> MSVPSLEYQKQYIYSMQKSQCSIQNQSINIIADEQQAPQESYLSRKCQRHLFETKCVQLELGLNGDYSLSNNSLFIQNNNTVFDNLQQNTESNIKQTNRSNKERYETQIFEQHPIIKNPKNDQVSSIMNEQEQKKFINTDENVQQTAQVSKNSKQSFKNGIQQVQTLSIDKSQASIREQKKISDCNLDKQFIKGDSRLDESSKIPSKCCGWIPEDIIFENNIHQLNKKVTLVAKNNFSDSKIQNHKEKKYQQNFQKAAEIVNRLLNTSMNRIMRVRQHVRNFIMLLKLRYLNRKIDDLTDRDYASINDLSNFYKSHKKKRNSKAFMKHFNFVIKLSQKLPIFMPTDTLRVVWDVILVLFTYIFLYFYSILMFFNQDNPDTEFIKEFYFCTFFIFLIDVLVNFNTAFFNKDLIIINRRQIAKQYIFSTVFFTDFVSLIVLGIKVIKRSNFIVYNPNHNLLTYCFNMLIFFKVNGISSKKKGFDYVFTLKESEKHVIKLINQLFSVITVAHLAAIGWYFLGILQVVNDNQTNWLVKLNISEGVYYQKYIYSIYWSITTMTTVGYGDISATNYGEALYISIVMLLFSCVFAYSINNIGFILQEIEKSSKQLNDKITTMQRYLNRKKVNISLKSRIRHYLSFLAQEQRDRDKQAEDEIISILSNKLREEITVEINSKILNKFNIFSSNFSKQTLDKLVFKMTEVLINPNEIIFREEQNDDMSIYFIQSGVIEVYQQSVQKQDKVTVIQTLTDESLFGEISFFSGLSRKASARSINLSTLYKISREDFIYIIQENNEDYERFKMIQEQIVFQGELPLLHVECYNCKKIGHISSSCPKTHQIFDKQFIIL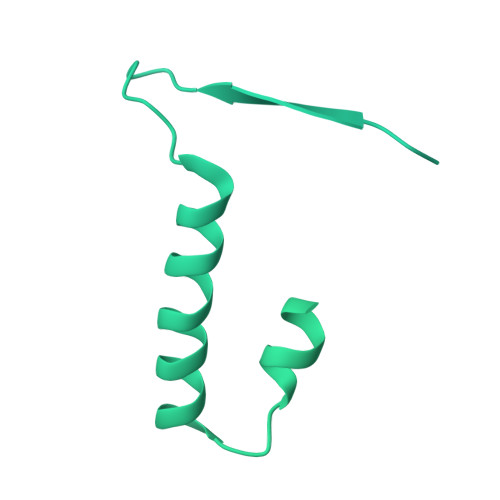REIYSSFQQRIFFDRTRYKNNLKPLNLIQDNQNVCKILKQNLQDDNISIEIMFDSCNRYTGSSYYNSEDLEDDEYGQCDEYATSSNSQTNIDNFSNKSSLNNIKNNALQKKKTMKKKEVSKKYLDNNQICENISSILNSDQYCNSQKVISNNINDNLEIKKSYVKSFNLSNRQKSLDDFEKIKSSQNLEQNNNFNNSDIQHSKSQIQIKADSEQFQQNIKAYSQTNKNEVDGDQEQSNISQIFKKRKSQKQQEQINNTNTDIKLQTEYPKQQARFSSTSGSTLQSQQLKMPSQKVQDELQLNINQNLKGQEFNINQSNKRVSTLLNQISNNHNQILKNCTEQTNYRNSIDQILLQGILVNNLIQSHSSQNILPIEQSFKYLKKADGDLEKKKNSILLQNFSLNNNKSSINITKEFIEDQAAVSHKNLSQIKTKQSIGKSSILNALSNINNIDGNTNDLNNKNNNSKLLQAQNSQITNGNQLQIVDRLSKLLLNPQLPLLLKLTSVGMSFREMNSINSNNAMDMFDKMHNFKKFFPHNNIENVLNKLKLLQLELKKQKKQKQINKPRRQNILFFRYYSNCGSQVHDNLKLLQQEFNIDDYRPTYLSYGVSKRRGQQFPCNKHNLTLYF>[2x]AVSLDRTRAVFDGSEKSMTLDISNDNKQLPYLAQAWIENENQEKIITGPVIATPPVQRLEPGAKSMVRLSTTPDISKLPQDRESLFYFNLREIPPRSEKAN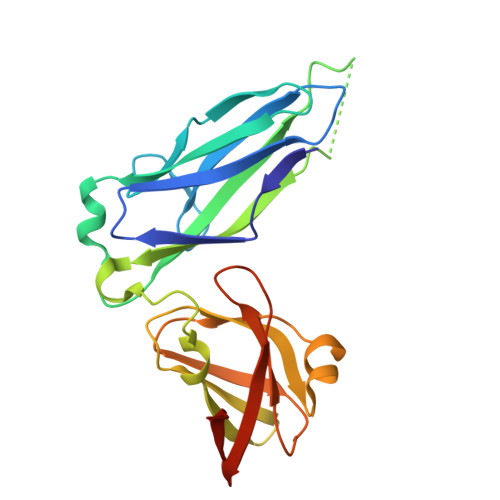VLQIALQTKIKLFYRPAAIKTRPNEVWQDQLILNKVSGGYRIENPTPYYVTVIGLGGSEKQAEEGEFETVMLSPRSEQTVKSANYNTPYLSYINDYGGRPVLSFICNGSRCSVKKHHHHHH> SAVEV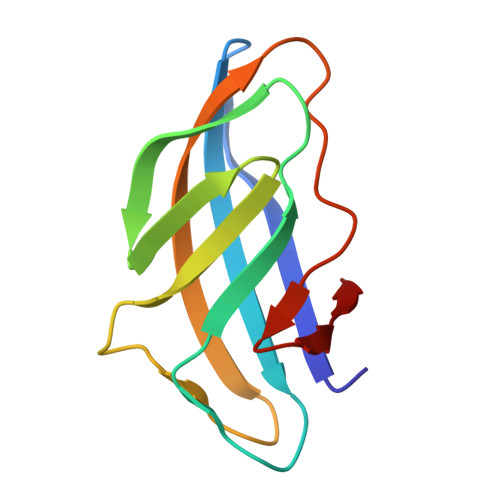TYAITNSWGSGASVNVTIKNNGTTPINGWTLKWTMPINQTITNMWSASFVASGTTLSVTNAGYNGTIAANGGTQSFGFNINYSGVLSKPTGFTVNGTECTVK> MELKNKKLSLWEAVSMAVGVMIGASIFSIFGVGAKIAGRNLPETFILSGIYALLVAYSYTKLGAKIVSNAGPIAFIHKAIGDNIITGALSILLWMSYVISIALFAKGFAGYFLPLINAPINTFNIAITEIGIVAFFTALNFFGSKAVGRAEFFIVLVKLLILGLFIFAGLITIHPSYVIPDLAPSAVSGMIFASAIFFLSYMGFGVITNASEHIENPKKNVPRAIFISILIVMFVYVGVAISAIGNLPIDELIKASENALAVAAKPFLGNLGFLLISIGALFSISSAMNATIYGGANVAYSLAKDGELPEFFERKVWFKSTEGLYITSALGVLFALLFNMEGVASITSAVFMVIYLFVILSHYILIDEVG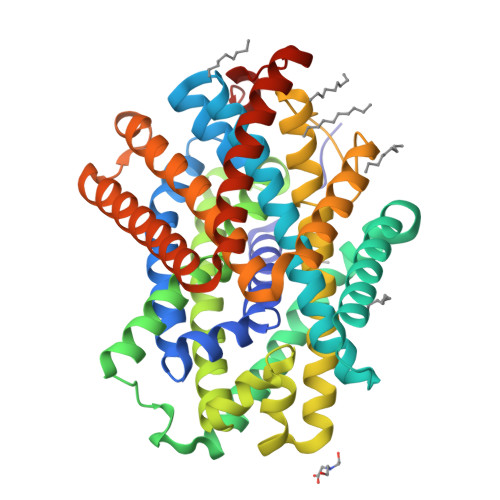GRKEIVIFSFIVVLGVFLLLLYYQWITNRFVFYGIIATFIGVLIFEIIYRKVTKRTFSNNMYVKSLESSGLVPR> TTLKDLIYDMTTSGSGSGLPLLVQRTIARTIVLQESIGKGRFGEVWRGKWRGEEVAVKIFSSREERSWFREAEIYQTVMLRHENILGFIAADNKDNGTWTQLWLVSDYHEHGSLFDYLNRYTVTVEGMIKLALSTASGLAHLHMEIVGTQGKPAIAHRDLKSKNILVKKNGTCCIADLGL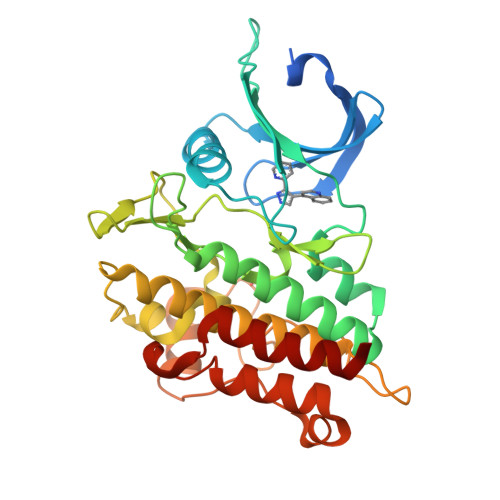AVRHDSATDTIDIAPNHRVGTKRYMAPEVLDDSINMKHFESFKRADIYAMGLVFWEIARRCSIGGIHEDYQLPYYDLVPSDPSVEEMRKVVCEQKLRPNIPNRWQSCEALRVMAKIMRECWYANGAARLTALRIKKTLSQLSQQEG>MRGSHHHHHHGMASHMSSKLVLVLNCGSSSLKFAIIDAVNGDEYLSGLAECFHLPEARIKWKMDGSKQEAALGAGAAHSEALNFIVNTILAQKPELSAQLTAIGHRIVHGGEKYTSSVVIDESVIQGIKDSASFAPLHNPAHLIGIAEALKSFPQLKDKNVAVFDTAFHQTMPEESYLYALPYSLYKEHGVRRYGAHGTSHFYVTQEAAKMLNKPVEELNIITCHLGNGGSVSAIRNGKCVDTSMGLTPLEGLVMGTRSGDIDPAIIFHLHDTLGMSVDQINKMLTKESGLLGLTEVTSDCRYVEDNYATKEDAKRAMDVYCHRLAKYIGSYTALMDGRLDAVVFTGGIGENAAMVRELSLGKLGVLGFEVDHERNLAARFGKSGFINKEGTRPAVVIPTNEELVIAQDASRLTA[4x]

Acetate kinase catalyzes reversible transfer of a γ-phosphate from ATP to acetate in the presence of a divalent metal ion. In the present study, we report the biochemical characterization and structures of S. typhimurium AckA (StAckA, NCBI accession: NP_461279.1, residues: 400, molecular mass: 43.3 kDa) in two crystal forms at 2.70 Å (apo, Form-I) and 1.90 Å (citrate-bound, Form-II) resolutions. StAckA protomer consists of two domains with characteristic βββαβαβα topology of ASKHA superfamily of proteins. A cleft between the two domains forms the active site pocket of StAckA.

Structure of Form-I StAckA determined in the present study represents the first report of an unliganded as well as mesophilic AckA. The asymmetric unit (ASU) of Form-I StAckA crystal consists of four nearly identical protomers, as indicated by the low root mean square deviations (rmsd) of corresponding Cα atoms (0.43-0.84 Å for >350 target pairs). The four subunits of StAckA present in the ASU are further organized as two dimers resembling the dimeric structure of the archeal enzymes. The subunits of a dimer are related by nearly perfect non-crystallographic two-fold symmetries. The accessible surface area (ASA) of an StAckA monomer was found to be 17,920 Å2 and upon dimerization approximately 3,061 Å2 (17% of total ASA) per subunit gets buried. A total of approximately 81 residues (20% of total surface residues), of which 23% are polar, 53% are non-polar and 24% are charged, contribute to the interactions at the interface leading to approximately 23 hydrogen bonds and 8 salt bridges. There are also a few water-mediated hydrogen bonds between the two subunits of the dimer. This analysis indicates a stable dimeric interface. The analysis revealed conformations of StAckA that were similar to both the open (Cα rmsd: 1.15 Å) and closed (Cα rmsd: 1.23 Å) states of MtAckA subunits, and in conjunction with fluorescence studies, suggests that StAckA is also compatible with the inter-domain movements as observed in MtAckA. It is possible that the structure of Form-I StAckA protomer represents an intermediate state in which the active site is accessible to the solvent and ligands. Intriguingly, examination of Form-I StAckA as well as other structurally known members of acetokinase family revealed a similar cavity at the dimeric interface.The principal constituent of the protein deposits is one of the most abundant proteins in the extracellular matrix (ECM) of the human cornea, transforming growth factor-β–induced protein (TGFBIp). The function of corneal TGFBIp is elusive, but its ability to bind both integrins and ECM molecules indicates a role in cell adhesion. TGFBIp consists of an N-terminal CROPT domain followed by four fasciclin 1 (FAS1) domains (FAS1-1, FAS1-2, FAS1-3, and FAS1-4). The X-ray crystal structure of wildtype TGFBIp reveals an elongated banana-shaped molecule with the five domains arranged like pearls on a curved string.

Lattice corneal dystrophy (LCD) is characterized by the appearance of amyloid plaques. In contrast, the asymmetric unit of the A546T structure contains two molecules, and the unit cell parameters are not related to those of the two other mutants or the unit cell for the wildtype structure. Crystal packing contacts shared by R124H and R555W offer an explanation for their aggregation phenotype, whereas the enhanced susceptibility of A546T toward proteolytic degradation was not immediately explainable from its structure. The low resolution of the data prevents the identification of detailed structural changes induced by the additional methyl and hydroxyl groups of Thr546. Nevertheless, a comparison of FAS1-4 domains from the structures available suggests that the overall location of the α5 helix–containing residues Arg553–Gly560 is altered by the A546T mutation. The significance of this difference is difficult to evaluate as the electron density for the α5 helix is weak compared with other parts of the structure, especially in chain B of the A546T structure. However, an analysis of residue B-factors (i.e., temperature factors) in all available TGFBIp structures suggests that large regions in the FAS1-4 domain, particularly residues 540 to 575, have higher average B-factors than expected in the presence of the A546T mutation. Elevated B-factors in a region of a protein usually correlate with higher mobility or multiple conformations of this region. If the elevated B-factors reflect a higher mobility or conformational heterogeneity of residues 540 to 575 in vivo, this would explain the phenotype and the increased susceptibility to proteolytic degradation. Three cross-links connecting the FAS1-3 and FAS1-4 domains were exclusively identified for A546T. Wildtype and GCD mutants were very resistant to proteolysis by chymotrypsin, whereas chymotrypsin readily degraded P501T, A546D, A546T, and V624M associated with LCD.

>GPNVCAVQKVIGTNRKYFTNCKQWYQRKICGKSTVISYECCPGYEKVPGEKGCPAALPLSNLYETLGVVGSTTTQLYTDRTEKLRPEMEGPGSFTIFAPSNEAWASLPAEVLDSLVSNVNIELLNALRYHMVGRRVLTDELKHGMTLTSMYQNSNIQIHHYPNGIVTVNCARLLKADHHATNGVVHLIDKVISTITNNIQQIIEIEDTFETLRAAVAASGLNTMLEGNGQYTLLAPTNEAFEKIPSETLNRILGDPEALRDLLNNHILKSAMCAEAIVAGLSVETLEGTTLEVGCSGDMLTINGKAIISNKDILATNGVIHYIDELLIPDSAKTLFELAAESDVSTAIDLFRQAGLGNHLSGSERLTLLAPLNSVFKDGTPPIDAHTRNLLRNHIIKDQLASKYLYHGQTLETLGGKKLRVFVYRNSLCIENSCIAAHDKRGRYGTLFTMDRVLTPPMGTVMDVLKGDNRFSMLVAAIQSAGLTETLNREGVYTVFAPTNETFRALPPRERSRLLGDAKELANILKYHIGDEILVSGGIGALVRLKSLQGDKLEVSLKNNVVSVNKEPVAEPDIMATNGVVHVITNVLQHHHHH[2x]>GCRLRSQLVPVRALGLGHRSDELVRFRFCSGSCRRARSPHDLSLASLLGAGALRPPPGSRPVS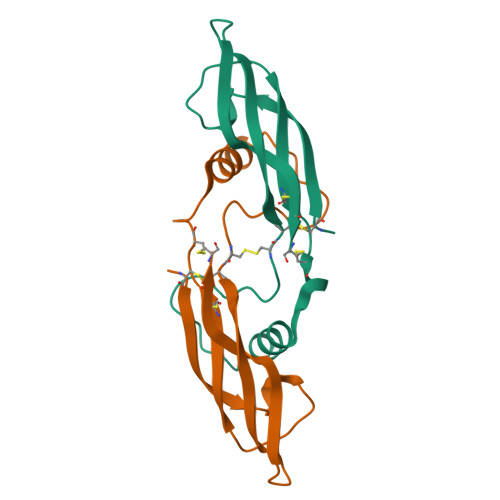QPCCRPTRYEAVSFMDVNSTWRTVDRLSATACGCLGHHHHHH[6x]> MASATAPAAAVPTLASPLEQLRHLAEELRLLLPRVRVGEAQETTEEFNREMFWRRLNEAAVTVSREATTLTIVFSQLPLPSPQETQKFCEQVHAAIKAFIAVYYLLPKDQGITLRKLVRGATLDIVDGMAQLMEVLSVTPTQSPENNDLISYNSVWVACQQMPQIPRDNKAAALLMLTKNVDFVKDAHEEMEQAVEESDPYSGLLNDTEENNSDNHNHEDDVLGFPSNQDLYWSEDDQELIIP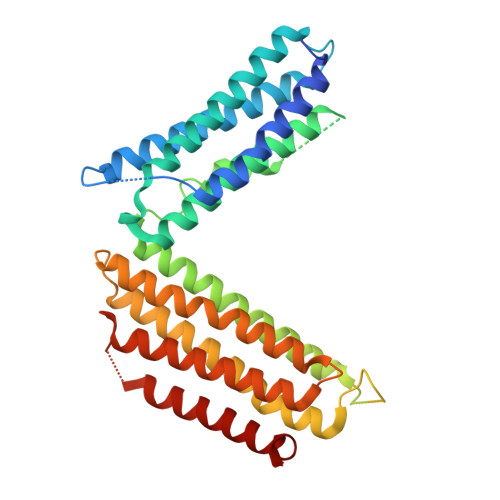CLALVRASKACLKKIRMLVAENGKKDQVAQLDDIVDISDEISPSVDDLALSIYPPMSHLTVRINSAKLVSVLKKALEITKASHVTPQPEDSWIPLLINAIDHCMNRIKELTQSELEL>[4x]FSCNVDGGSSIGAGTTSVYVNLDPVIQPGQNLVV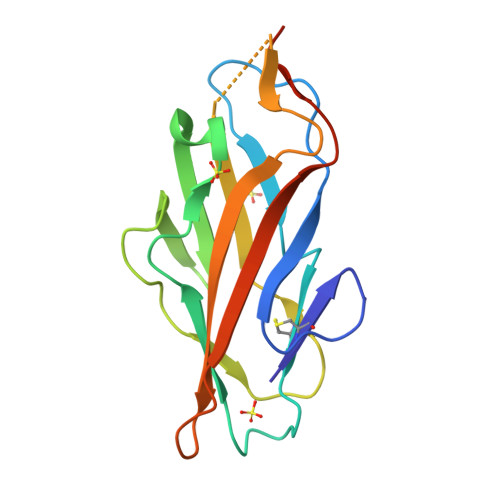DLSQHISCWNDYGGWYDTDHINLVQGSAFAGSLQSYKGSLYWNNVTYPFPLTTNTNVLDIGDKTPMPLPLKLYITPVGAAGGVVIKAGEVIARIHMYKIATLGSGNPRNFTWNIISNNSVVMPTHHHHHH> EACGYSDRVLQLTLGNSTITTQEAANSVVAYGRWPEYLRDSEANPVDQPTEPDVAACRFYTLDTVSWTKESRGWWWKLPDALRDMGLFGQNMYYHYLGRSGYTVHVQCNASKFHQGALGVFAVPEMCLAGDSNTTTMHTSYQNANPGEKGGTFTGTFTPDNNQTSPARRFCPVDYLLGNGTLLGNAFVFPHQIINLRTNNCA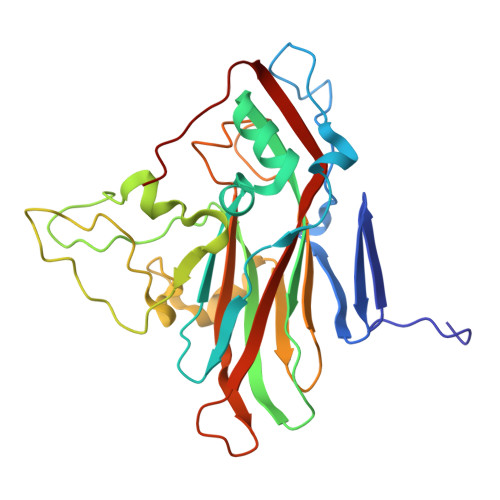TLVLPYVNSLSIDSMVKHNNWGIAILPLAPLNFASESSPEIPITLTIAPMCCEFNGLRNITLPRLQ> MKNELICYKQMPVWTKDNLPQMFQEKHNTKVGTWGKLTVLKGKLKFYE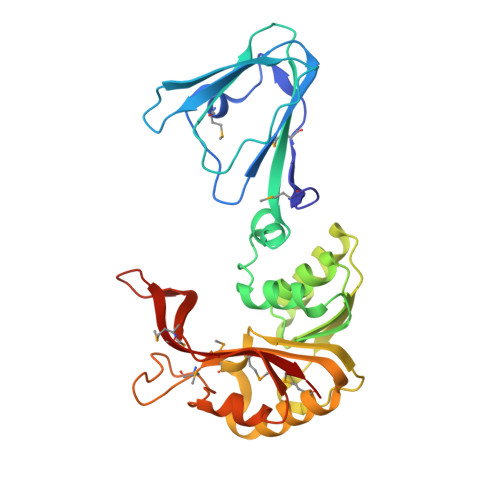LTENGDVIAEHIFTPESHIPFVEPQAWHRVEALSDDLECTLGFYCKKEDYFSKKYNTTAIHGDVVDAAKIISPCKVLDLGCGQGRNSLYLSLLGYDVTSWDHNENSIAFLNETKEKENLNISTALYDINAANIQENYDFIVSTVVFMFLNRERVPSIIKNMKEHTNVGGYNLIVAAMSTDDVPCPLPFSFTFAENELKEYYKDWEFLEYNENMGELHKTDENGNRIKMKFATMLARKK>[4x]NVAPKFLANMTSVILPEDLPVGAQAFWLVAEDQDNDPLTYG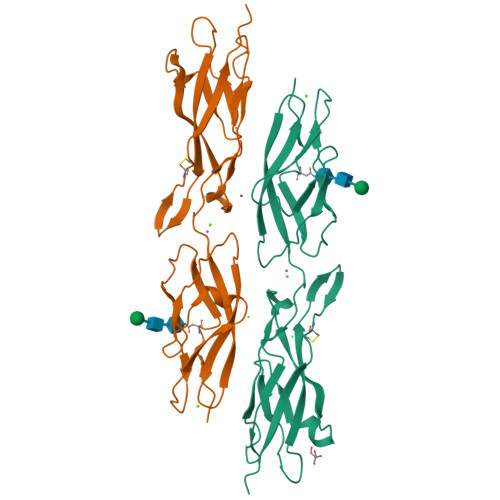MSGPNAYFFAVTPKTGEVKLASALDYETLYTFKVTISVSDPYIQVQREMLVIVEDRNDNAPVFQNTAFSTSINETLPVGSVVFSVLAVDKDMGSAGMVVYSIEKVIPSTGDSEHLFRILANGSIVLNGSLSYNNKSAFYQLELKACDLGGMYHNTFTIQCSLPVFLSISVVDQPDLDPQTVPRARDPPVGGHHHHHH> MNSLLFVYGTLRKHEKNHHLLAQSACINEQARTKGSLFAAKEGPTVVFNDED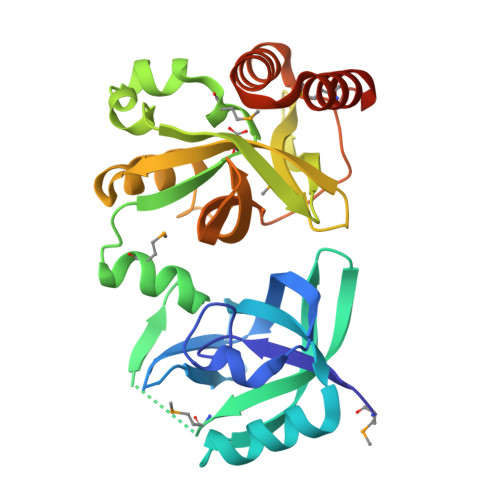EGYIYGEVYEADELCIHKLDQFFQGYHKQTVFVETDVGIKIALIYFMNKDGCAGFTKISSGDWKEHQMISKSKNPIYYFAYGSCMDNARFQKAGVDHYFQDPVGRAVLKGYTTRFTLKREDGSRADMLEDGGTTEGVLYRIPYSALSYLYKREGVESLTYRPAFVDVEAGGRHYKDCLTFLVLQKEAEIAPPQHYQIEIERGAELYLSPEFTEKLKRHMNSLPKGLEHHHHHH1-benzyl-N-{5-[(6,7-dimethoxyquinolin-4-yl)oxy]pyridin-2-yl}-2-oxo-1,2-dihydropyridine-3-carboxamide 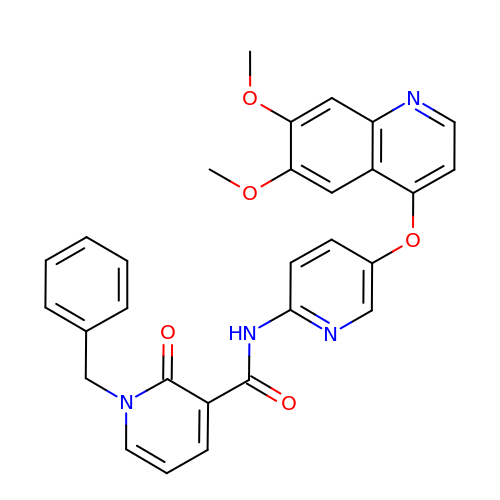| C29 H24 N4 O5 | MIRAJAFOEINWJO-UHFFFAOYSA-N> RETLQAYDYLCR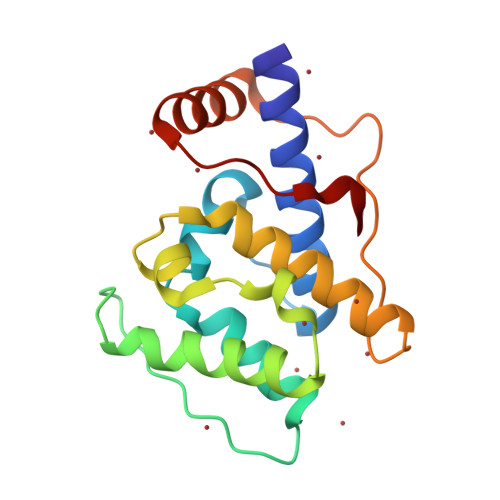VDEAKKWIEECLGTDLGPTSTFEQSLRNGVVLALLVQKFQPDKLIKIFYSNELQFRHSDNINKFLDFIHGIGLPEIFHFELTDIYEGKNLPKVIYCIHALSYFLSMQDLAPPLIKSDENLSFTDEDVSIIVRRLRQSNVILPNFKAL>[4x]ADQRVRDIMIPRSQMITLKRNQTLDECLDVIIESAHSRFPVISEDKDHIEGILMAKDLLPFMRSDAEAFSMDKVLRTAVVVPESKRVDRMLKEFRSQRYHMAIVIDEFGGVSGLVTIEDILE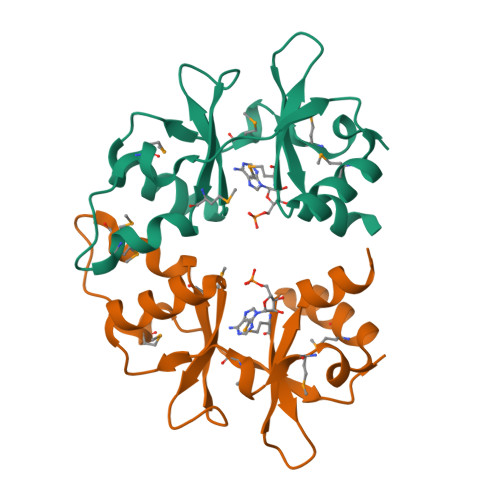LIVGE>MLNQSKILTLQAYDPAKVLVFIGGQRVSGFAADTKIVITRNNDNISVHAGVDGEISNALSRDNTGVMTLSLQNTAKWNGYLAQWQRQANVTGLIYLPVQVEGSQGLSLNTIGWIQKQPDLSYGTEVGQMDWEIGVLDAWLSPDQIQGIAAGITGLLGLDQ[162x];>[12x]MTNEQVIELVRVLLGGITTEEISDQTIIFFWTKWKLTYDLDNRPEKIPAALYNTVVDCVRWLIVQEVSSGNSSIRERFEKIGDETISVKGGSSWESWKDFLDWLELNPDYIDPSLAFNSSLVIIGGVRKDEFFRVKNNPNSYNGFMEQGVYPTPAIPKQSAWPCTAARRSPWMVR;>[6x]MARAYSLLSSRNRLIPRVEVQCRKREWVKTDPDSPFLNGGREVLYTPFTAVECTVQPMRGKAIRDQNNQLMIGGEEDYDSYTVYSETLLFRAREGTEHLSDQMLLPDSGGGQTWFTVMKADMYPSSGVPRYRYYLIAVPVGTEGGL;>[6x]MALPLDFTNSDVVMGALTKAVGRLCLDVTGYDVVEADETIPKPEGPYILVDLSLLTPLDWATNEVVDEDGVVHTAHNYTASYTLTAYRGKPHWALSRVHQAFGLPFLREKYFPTGSPYAYSSTSNIARMRVPLNQQMFENRARTIVTFNATFVEKDLGTFEDIEHIIIGIDVDNPSGPPIGIGADYDKGVKPGGDDPGLPPKPNPPIVYHDAIAQVCMATPVIDKPALISDKTGE;>MAEYQDKVVDVEVSLGTQPIDTVGFETPMFLAMHGNFPERIRFYVSTAGMVADGFAVGSPAYQFATNAFAGNFAPQRVAIGRMSIDSSKVDFTGTTNTEQVVVNITLNKVVKAVKINVLPGNTPAQIATALADAVTADADLTGKATAVATGTYVTVTAVSPNVVSVGKGAGVYKIVNESSETVATVLPSVIAENHNWYFLATEARSDADIVAAAEFAKANYKLHIYNSTDVDAYAPENSAASVFDTLKSLSYDSLGTSDAGADVDFTEGSVIGAMAANDPSYGDSLHLKTMPGMVPFAGSDTQRSNAWSRNANIYRGLYGGGSYIEGKTSSGQYVDVIRFSHWVKFRMEESVFAYMKRRSDMGLSMKMSDEDLPVLKSVLMNNPINIGIRNGGILTGYDTENKVSYDPTIIIPKRANIPTNDLAARILRDVKVELVYNNSLHYVKIRASVVLDRPAGQSTNAQTPMSSSAVGV[162x];>[12x]MSRKRNRNRSVQVAKATSEQLNVSRMRMSEQGTFALAKVQVDSERMKAEEIRWPHLIGTAESMKQDATVATGLDMLYTFVEKAFKDFKVIPGESEESKKAAKFIEYCLKNMEGQTLRQFARDAATFNEYGLSVVEKVYTQIAVGEYVGKYKVKNLAFRPQASLSRTNPIVYNSDGSAIVGIKQSLSAFQNYTASEIGVGGVSTRMSDVIIPISRVMLMNTGGSSSQALGVSPLVGCYRAWREKILIENLEVVGATKDMGGVIELKIPSQILNKAAMDPSSPEADMVRGLMSDAANAHSGEQSFFMLPSDTKDNAPQYSMTLKGIDGMGKQYSTAQLISDRKKSILDRLGAGFINVGNDKGGSYNLSESKQTIHTQFVQRVNEIILEALNENLLPQLLALNDIRLPETEMPYVKAGEIVDVDMEGFSKAIQRIGAVGYLPKTPKVINRVLEVLGIDEKIEEDISQEELMKLLGEDTSRAGDGMTKGSSGNGTGKISASRDNSAANLDN;>MAKAHVATLEGNYSDIVLGRVVAFGDTGWNFKEVDMTFIADDADADSKTTLFAGVLVGEDGTPATAAAGVFGVLVDRKVLPGVDHYIGVFEPGEKVPMVLAVRGLTLNQLKLKYADGTAIDAAGIQALEAQGNQVTDKIVGTQFIGSVL[780x];>[775x]MQNGDFQILDYTGLISTMPRVDTLLQSMNLFTEHFGRTTVARIERLDDGAGDIKAVQRGGVRQHLANDRKKIVNLNIPFFPLDRSIDRADIQNFREFGTENAPATVDAEVQRHMARIRRSHAILKSKAMYAALKGTSWSPDDPVSDYNYYDVWGATQTTADVDFTKLGVDPIEVLEAEARAHIIDWAGDNGDNYEIVVLASRQWFSALIAHPQVTGAYSQYPSTQEILRRRLGGNANNRIFEHKNILFIEDISGNIPAGEAYIFPRGISRMFEIYYAPSDTLRDANQAAQELYVFFKESNYLREAKIESETSFLTVNNRPELVVKSTGKFTA;>MSSNTDIIALLSSDADKAVDQIIEDSKRLHIVVNGTGTEQAVAEDGSLLPSVRKALIDNLYFKTPPLPWRNGGSVNEFNQLYSFTDVSGNTTWWYAPGATVSNPVVMRDSPINDGKFKVFLDKTNIADIYAPLNSPNFVGNPRVPTPAPGDNSQSIPTTGWVQSEMEGLEDLIISSMRGEFENITVRNDAILQDTYINGEFIVTSDKLAAANTEATFRRIRMVGTGTTGTAATEIAFEQNTTPPPGVSTKTNIKPFAVSTGILTVDQINGKAAQVGDVAVSTDSLNVDGYMRGDYLHLEGNNRNTAGRPQLIVDGIAEIETLRVTGTIEGVKADVDGLDIHPRSVIVDEGLTVAKDTTMTGKLTVGGTTKVGNLEVTGTLSGVAISVDGKDIKPRSVNTGNLVATGDVQISGTTTATGKITTQDLEVLGTLTANLDLSGSDLSVDNINVAQTATITDLVVTGTTTGVKGDVEGEAIAPASVAATGTVSAASMSTTGNMAVGGNLTITGDFRPASVAGQDTPRLVVQGDSDLQGDLNVSGTITGVVDLTAQDINMNSLGLAQGLTAGGGITSFSTVKGVNGVFGEGSTAPGAIGLQSMTNAKVATDLLVGEDLRVEGDTNLFGNLSVTGTITGNMNFSGKTIAPATVNATTVTATNLTVTGTIDLTDSPIVAQEITATNVEATGKMVAGKYSTTPKTANATTATFTPDGTTSIYNVNVQADTEVQAPAGLLSSGKGESIFIYFEQDTTGHAVTFSSAFVVHNAATVSNAANSITIANLVYRGTGPLIDVFLTGR[18x];>[6x]MATQFKDLLLDPLTGDLDFGTPGDRGMRLALTNQLSLRQRLYLRFAIWAGDWYFDETFGFPYRTFVGKKTVKAVLDGRIKSEVRQEPDVLQITDFQSTMDVVSRSYKCFFTVVTAEGEEISLAFVGEDEYQYPTPPESNVQLCGDEGVIINFKNKLYYLINFRLPKYGDSTWVNSWK;>[6x]MAVNNNSISPAQQAQADKRARDAAAAKRKQDTEVSNAKSREDIQYTMFVSGLRRGRLNEFERKNRTDDLAILFDSVTTHTYTKDYNKSSYAVESKAKASDHVTTQDGKFTFSGTVTDSPYLIDPRNMIDRDTDKENPMLARRPAKAIEILELIADSHQLVTLVTEDNILSNYVITSFQVDRSSEAGSSINVQVTLEEFRFKMVNKTVMARTSDPKKAKNANTGTKQTAEDGAVDDSAKQKRQTPYIGKNAETKERWENAAIGTTDFSGKPGAKLPFDPSDLMRK;>MANTTERTVVRTFDFELSGYPDETFRVVLDSVTYELRFMWNERDESWFMSLGDIGAQRPTITSKLTCYSDILAPYRYLDNVPDGNLYLWPLGDIRTRAGRFNIGPLKGIQMTYSSLIEDVEDIE[6x];>[6x]MVEEIVLKDVNHIHPLPDFVRGGFDYVPSDIFSGKENFEQTLRILLERLEFIDQKMVELAELRTTLNAEDAILDEIGRQLGIYRNGLNDPEYRAVIMILTGNNSKSGTRADIIATLKQLFGEDGVTTYKGYNYRLDINIFNTCMEVTDILPEIIDMLPLVTHLRVVENQGYPFGFNGDTQAFGFASVYDSGRTGEGGMSTLIYVSDDEEDWSFT;>MAENYGLTGSGFNLPPMDDLVQETKKTFKSAFGEDFNTESNSVADKLIQIFNEREYQLWLLMGSVYYAQTMQGAEGIYLDDLLGKRGIYRLGKTRSTGTVVMTIDSSVPYNMIYSAATYTIDTDYELSSDVQVAGNIVAQLIKGTDLSVGTYRLQIQNTTDQSVKTLSLNLTATSGQPLITFFGQIKDFIVNNTILSNQDRIWIDSTEGALYIGYDTNKIMIGLSSRVDFRTNPMAGTRSISMDVRSIEPGYISRDVHSVRSINPTPGGFVDIDNLSAFIDGSDVESDNEYRIRAATSISEGKATRPAILAALLNKVEGIEKVRIFNNNTDKTNSLGIPPYRFMVVCYGGGTAEISQVLYDTIATSNNTYGDTFYDITTEDDQVERIWHTKAAARQLAIRVRYRGRPLSLTEETAIANGLATAVNGTMIAGTLYNVRLVGTVMSSTSPDRFTQVYVDIKNKGQPDSAYVNTDVTASTTQVLSLELEDVIFSQIV[12x];>MAASGNVVVTRTTNRVTFETDKASYARAVKQIRQVGKEWEKASDAISKPKKDPAKAYDKSAQQMRLVNKRLAETRAREEKRASERSIALARREAKAKEAIARVSAARIKQQVQQMTSPRAGMSEMKKFYQQQEREAKKANRKATIGMNAASRPMNVTRINSAPLSPRGGQGTGMVGDPNKVYNPELIAAQNRAMAGRIRSQSQAQDRKAKAEARQRAAAAARAARIDDVMAQQRIRLSSKYGRSYEGRLGRDGAGQGIQDLNRQFRAGTLSAGQYRQSIQALERQFRSAQANAGGFGAALGDIRSQLLNAGAAYGVFASGASVLKQGQFFQGMEATMSMVSDSSEEAGQRIKFVKDQAYRLGLDLKIASQGYTQMAVNSAGILSKAQNDDLFKGFSEFATASQVDPVKFQRGITAIGQMMGKGQVMAEELKGQLAEGIPGSLQVFVKAAQEAFGDTTIDVEKLMDMMQKGELKAAKILPFVGKYFAEAARKGGALPKALESNRVAMQRLSLTWIDFQNQIFQGGFGEQMTRVFRDLATILDSNGELATNLGAFFGNVIEGFWDMVTEIHDDFVLLDRIVSYYTEKLGYQGDLLKEVFDWAGYAIGIGIFVGGLNKIFKILTKIAGLRTALVGVRQAMGGAITRGGVTNGAGLGGGAGAAGTPGASRTASFLSKWKGLSKISKVGILGTLYSAGSMLNEQFIKRGDDKLADAGLDQETFQKEYGFMPKPVGLLDVFDKWFNKPRDLDAPTITAPGPGSGMAAQTGIPFPAPQKVEGDITIKIEAGELRNMVRAVVDENNQFNFNMLIQGGPN[3x];>[3x]MRAMERTYTLVIGRPVVIGEKPVNIEKFANTSKGDAYEIKDLHIEFNVKKDNSKEPNKGYVTVYNLSDEVVNYLSVNQRESLAVMLHAGYNGDEKLIFSGTVEYVEDDFPEETRTTKFILGDGTLNLTTATTARSYRKGTPVNSVLNDLIADLKLPKGRVIDFGNQTLQTSMAFTGNASQNLANLAKNTGSTFSVQDGAVYWTKEGSRFNNVMFEISEEGGMVGTPTPKQPSSSKKLIKAKAKAKSDEAEGKKPKAPSKKKKEHDIKEDVGMTVSTLLNGAILPESTVYLNTRYHKGFYKVAELTHRGGYETGDWITELGLVETRGELIK;>MAYADRYDAAFGIYISRFLRNNVHTNIRGKVVGVNYSGPSVDVQPMAYTEFPSGTTDRYPVIYDVPVLLPSGAGGKARLTMPIKPGDVVGLSFSERNEGDNNDQNTHQLFAGWAVTQIFTDGNSKAIHPDNVVLENDKAIITLKPDGDTSLQNPKVTVEALADGNVKISNGTGEFTMSPSGEIKGGNRGGSFTLQPSGQLMCNGARITTSGRIITANGVDMDDFYQKYMSHTHGGVSRGGDNTNPPN[3x];>[18x]MAKPKDPIYVWAAAD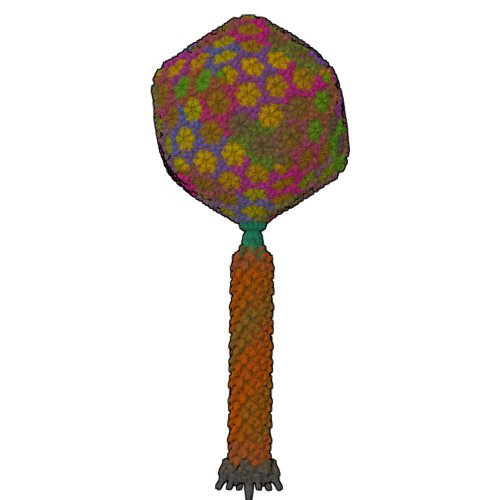VNLPGTGRPNKSKPIDDLLAKGYDKGQKPAAEEFNYILNMSSAWVNWIVNEKFPELEAEIARLLAELENRINQQLAVIRQDIAQLRQDVADLRRYVDQKVQELKQEIQGVRNDLNKLRQDFDAAITQVNGRIDDLEPRLVPIGAVIPWPGATVPDGWLECSGQVFNTGQNPKLYSVLGRNVVPDYRGLFLRGWAHGSDANDPDAGRALGSVQGDAIRNITGYFPADIGNSNFIGRYVGGAFRDDGSLTSGDDGTRSNEVRKYSFDASREVPVAAENRPKNIAVMYIIKTDQAQSSGGNSPTAIVVSPDTITNRIGYAVKATASVLPASISGQYPISWSTQNAAVATVDGSGNISLVGPGETNIIASISTGMNVVIRVTSYSVLTSISIADPGQITVTESKMLVVTKSPSSANEPLQFLSNNSGVAAVNDAGYVIGVSAGSATITVRGTLSGVSSTRAVTIIPEQVEESVQDNRLGAVGSYIPPSPSSNVMSWTFQAPQGCALTGIIVQENESNSGDNIGGVYYKPIQKKVNGVWVTITG>AAPDEITTAWPVNVGPLNPHLYTPNQMFAQSMVYEPLVKYQADGSVIPWLAKSWTHSEDGKTWTFTLRDDVKFSNGEPFDAEAAAENFRAVLDNRQRHAWLELANQIVDVKALSKTELQITLKSAYYPFLQELALPRPFRFIAPSQFKNHETMNGIKAPIGTGPWILQESKLNQYDVFVRNENYWGEKPAIKKITFNVIPDPTTRAVAFETGDIDLLYGNEGLLPLDTFARFSQNPAYHTQLSQPIETVMLALNTAKAPTNELAVREALNYAVNKKSLIDNALYGTQQVADTLFAPSVPYANLGLKPSQYDPQKAKALLEKAGWTLPAGKDIREKNGQPLRIELSFIGTDALSKSMAEIIRADMRQIGADVSLIGEEESSIYARQRDGRFGMIFHRTWGAPYDPHAFLSSMRVPSHADFQAQQGLAD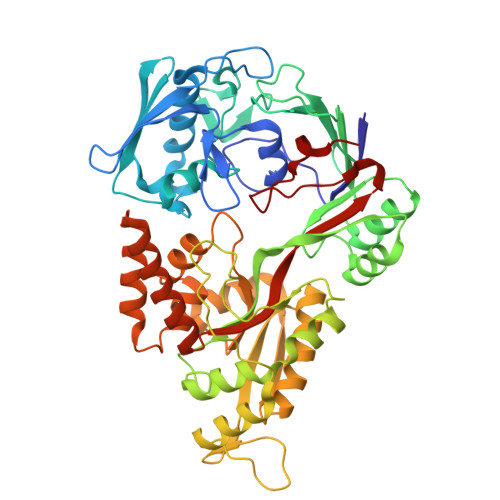KPLIDKEIGEVLATHDETQRQALYRDILTRLHDEAVYLPISYISMMVVSKPELGNIPYAPIATEIPFEQIKPVKP[2x]> MKKEKIDLFYGALLHDIGKVIQRATGERKKHALVGADWFDEIADNQVISDQIRYHMANYQSDKLGNDHLAYITYIADNIASGVDRRQSNEESDEDASAKIWDTYTNQADIFNVFGAQTDKRYFKPTVLNLKSKPNFASATYEPFSKGDYAAIATRIKNELAEFEFNQAQIDSLLNLFEAILSFVPSSTNSKEIADISLAEHSRLTAAFALAIYDYLEDKGRHNYKEDLFTKASAFYEEEAFLLASFDLSGIQDFIYNIATSGAAKQLKARSLYLDFMSEYIADSLLDKLGLNRANLLYVGGGHAYFVLANTEKTVETLVQFEKDFNQFLLANFQTRLYVAFGWGSFAAKDIMSELNSPESYRQIYQKASRMISEKKISRYDYRTLMLLNRGGKSSERECEICHSVENLVSYHDQKVCDICRGLYQFSKEIAHDHFIITENEGLPIGPNACLKGVAFEKLSQESFSRVYVKNDYKAGTIKATHVFVGDYQCDEIHKYAALSKNEDGLGIKRLAVVRLDVDDLGAAFMAGFSRQGNGQYSTLSRSATFSRSMSLFFKVYINQFASDKKLSIIYAGGDDVFAIGSWQDIIAFTVELRQNFIKWTNGKLTLSAGIGLFADKTPISLMAHQTGELEEAAKGNEKDSISLFSSDYTFKFDRFITNVYDDKLEQIRYFFNHQDERGKNFIYKLIELLRNYESEEKMNVARLAYYLTRLEELTDKDERDKFKQFKKLFFKWYTNNESDRKEAELALLLYVYEIRKD;> MTYKLYIMTFQNAHFGSGTLDSSKLTFSADRIFSALVLEALKMGKLDAFLAEANQDKFTLTDAFPFQFGPFLPKPIGYPKHDQIDQSVDVKEVRRQAKLSKKLQFLALENVDDYLNGELFENEEHAVIDTVTKN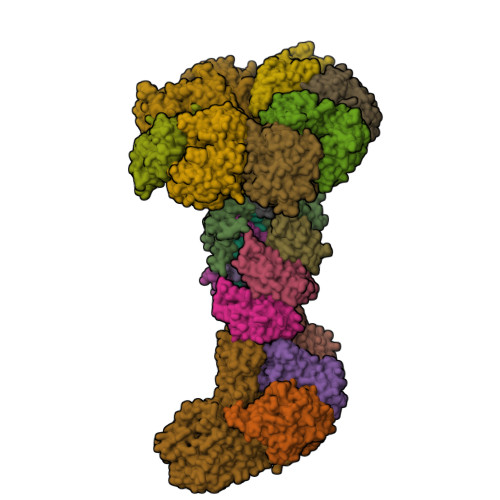QPHKDDNLYQVATTRFSNDTSLYVIANESDLLNELMSSLQYSGLGGKRSSGFGRFELDIQNIPLELSDRLTKNHSDKVMSLTTALPVDADLEEAMEDGHYLLTKSSGFAFSHATNENYRKQDLYKFASGSTFSKTFEGQIVDVRPLDFPHAVLNYAKPLFFKLEV;>[4x]MTFAKIKFSAQIRLETGLHIGGSDAFAAIGAIDSPVIKDPITNLPIIPGSSLKGKMRTLLAKVYNEKVAEKPSDDSDILSRLFGNSKDKRFKMGRLIFRDAFLSNADELDSLGVRSYTEVKFENTIDRITAEANPRQIERAIRNSTFDFELIYEITDENENQVEEDFKVIRDGLKLLELDYLGGSGSRGYGKVAFENLKATTVFGNYDVKTLNELLTAEV;>HHHHHHMAILTDENYVDKAERAISLLEKDNKGNYLLTTSQIRKLLSLCSSLYDRSKERKFDELINDVSYLRVQFVYQSGRNSVRVNRQTFFPVKDLVEKGQILEALKEIKDRETLQRFCRYMEALVAYFKFYGGKD[3x];> MKNDYRTFKLSLLTLAPIHIGNGEKYTSREFIYENKKFYFPDMGKFYNKMVEKRLAEKFEAFLIQTRPNARNNRLISFLNDNRIAERSFGGYSISETGLESDRNPNSAGAINEVNKFIRDAFGNPYIPGSSLKGAIRTILMNTTPKWNNENAVNDFGRFPKENKNLIPWGPKKGKEYDDLFNAIRVSDSKPFDNKRLILVQKWDYSAKTNKAKPLPLYRESISPLTKIEFEITTTTDEAGRLIEELGKRAQAFYKDYKAFFLSEFPDDKIQANLQYPIYLGAGSGAWTKTLFKQADGILQRRYSRMKTKMVKKGVLKLTKAPLKIVKIPSGNHSLIKNHESFYEMGKANFMIKEIDK;>[8x]MSIITDVYAREVLDSRGNPTLEVEVYTESGAFGRGMVPSGASTGEHEAVELRDGDKARYGGLGTQKAVDNVNNVIAEHIIGFDVRDQQGIDRAMIALDGTPNKGKLGANAILGVSIAVARAAADYLEVPLYSYLGGFNTKVLPTPMMNIINGGSHSDAPIAFQEFMIVPAGAPTFKEALRWGAEIFHALKKILKERGLETAVGDEGGFAPRFNGTEDGVETIIKAIEAAGYVPGKDVFIGLDCASSEFYDAEHKVYGYTKFEGEGAAVRTAAEQIDYLEELVNKYPIITIEDGMDENDWDGWKALTERLGGKVQLVGDDFFVTNTAYLEKGIAEHAANSILIKVNQIGTLTETFDAIEMAKEAGYTAVVSHRSGETEDSTIADIAVATNAGQIKTGSLSRTDRIAKYNQLLRIEDQLGEVAEYRGLKSFYNLKK;> MKNFKISSTYRAARKQQKTANRKSFYNDEGYMISPSEWADGVIKGLINPKNSWSNDHVKGYLPRVSPRSHWTKNGYREYLGIGKSRDIPEKEPEVIEMMDLELVV(3S)-3-(5-fluoro-1H-indol-3-yl)pyrrolidine-2,5-dione 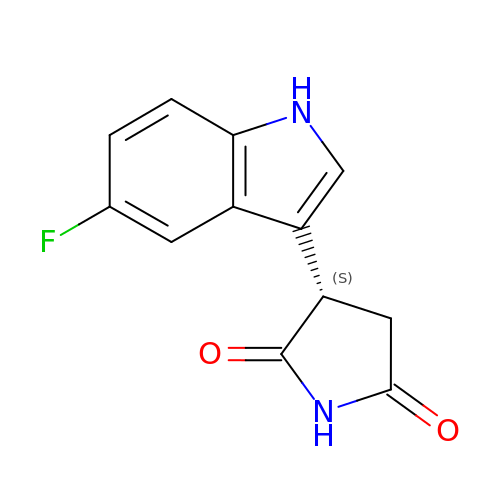| C12 H9 F N2 O2 | MXKLDYKORJEOPR-QMMMGPOBSA-N>[4x]HHHHHHGSMGYPVIVEATRSPIGKRNGWLSGLHATELLGAVQKAVVDKAGIQSGLHAGDVEQVIGGCVTQFGEQSNNISRVAWLTAGLPEHVGATTVDCQSGSGQQANHLIAGLIAAGAIDVGIACGIEAMSRVGLGANAGPDRSLIRAQSWDIDLPNQFEAAERIAKRRGITREDVDVFGLESQRRAQRAWAEGRFDREISPIQAPVLDEQNQPTGERRLVFRDQGLRETTMAGLGELKPVLEGGIH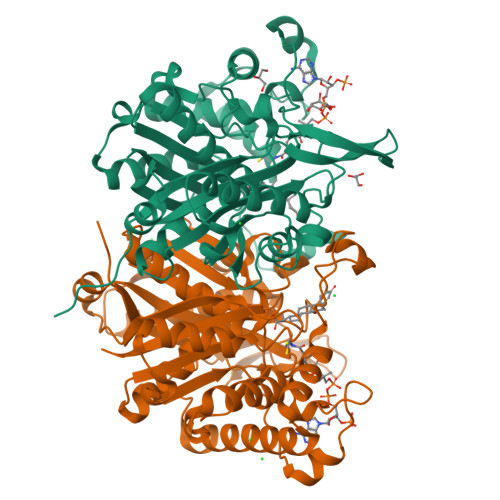TAGTSSQISDGAAAVLWMDEAVARAHGLTPRARIVAQALVGAEPYYHLDGPVQSTAKVLEKAGMKIGDIDIVEINEAFASVVLSWARVHEPDMDRVNVNGGAIALGHPVGCTGSRLITTALHELERTDQSLALITMCAGGALSTGTIIERI>[2x]GMEPNDSTSTAVEEPDSLEVLVK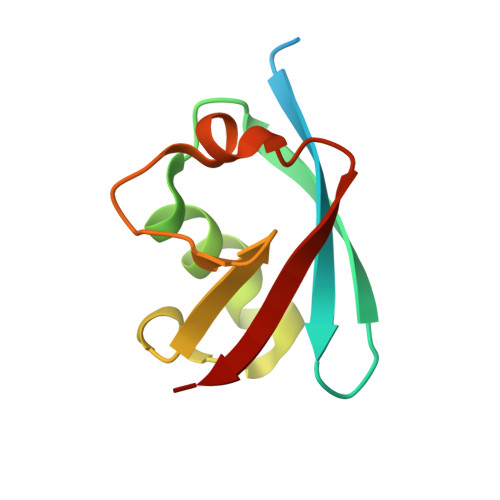TLDSQTRTFIVGAQMNVKEFKEHIAASVSIPSEKQRLIYQGRVLQDDKKLQEYNVGGKVIHLVER> MASRLLDPDTLVELEGVNGEWFDLTNGTEGIYLATEVTGLLDPPVKATYEEPGNFPGARYLNHRVLRRDLVFGVEILNDENDETWLRRDSAWRKAWSFKRDAKLHITTGESGHRYLKVRLFESPTTDMVTDPRGREVNITKMVVVAGDPFWYEDDVVYPIEVQEDTTFDPNPLPWPWPQPELPVEDIEITVPNANPTDNIIWPKWTLPGSSEKPAEPYIPGLPWLGAPKSPATLWTVPDYKLDLDEDEDPSLGTRRIRMPGQIGGLRVEEVQQIYIDGRPTGGTFKIGYGDEWTEPIAYNASPNDVRAALIALEGISANDVEVSLGGATNEVQTVRLKGGALGGTFTLSLGSETTVGIPFNASDADLQGALVGLDSIGSADVRVKSTKINEVQVVELVGEPTSGSFTLTLDGQTTAPIAYNATPATVAARIADLPNIDGNYVKVEGLNEWFHSPYRITFGEAQSQGVITDIISGIIDFIGGLFGGNASGKGVGGIDIDEMTGDVGTLSGGAGLDVQVTTEQDGDRLYVVSFQRAAGGLNLPQLVGNASGLEGDDLSIETATNVDGGRPYVVRFTDDLQGVDVPTMTVDTDDLTGGYEVGSRVVVLREGYTYPAENVVVDSDPREEQVSSESGSPIWERMNSVRFLHYIPPYTGEVTFKLSVSGAVPGQIATLRLPR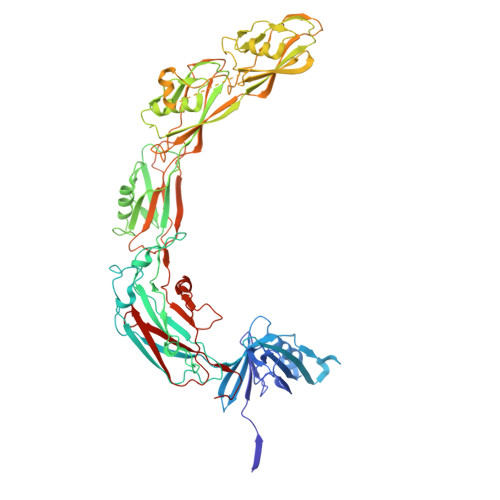AWSRPWGLE>SNAMTHLLETFEMSIDHQEDGLVVISMPVTDKVKQPFGYLHGGASIALGETACSLGS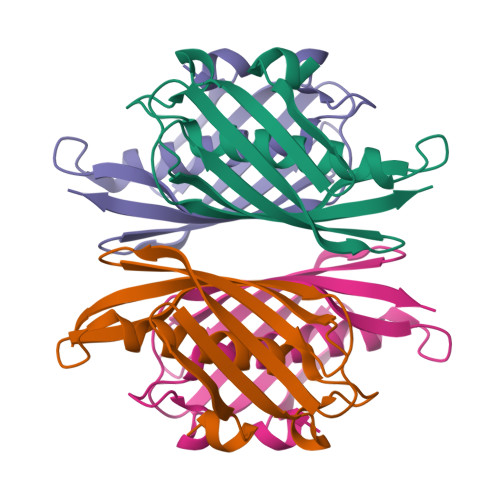ANLIDTTKFIPLGLEMNANHIHSAKDGRVTATAEIIHRGKSTHVWDIKIKNDKEQLITVMRGTVAIKPLK[4x]> TPTTFVHLFEWNWQDVAQECEQYLGPKGYAAVQVSPPNEHITGSQWWTRYQPVSYELQSRGGNRAQFIDMVNRCSAAGVDIYVDTLINHMAAGSGTGTAGNSFGNKSFPIYSPQDFHESCTINNSDYGNDRYRVQNCELVGLADLDT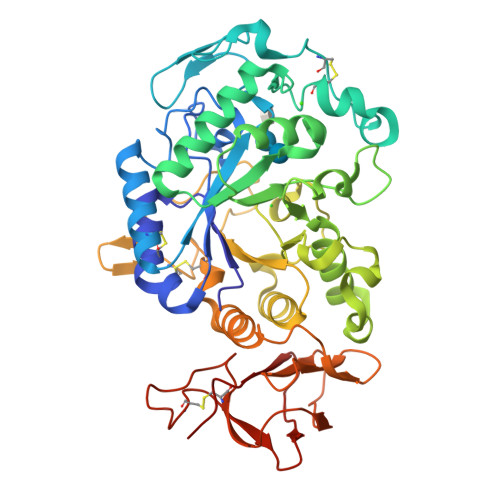ASNYVQNTIAAYINDLQAIGVKGFRFNASKHVAASDIQSLMAKVNGSPVVFQEVIDQGGEAVGASEYLSTGLVTEFKYSTELGNTFRNGSLAWLSNFGEGWGFMPSSSAVVFVDNHDNQRGHGGAGNVITFEDGRLYDLANVFMLAYPYGYPKVMSSYDFHGDTDAGGPNVPVHNNGNLECFASNWKCEHRWSYIAGGVDFRNNTADNWAVTNWWDNTNNQISFGRGSSGHMAINKEDSTLTATVQTDMASGQYCNVLKGELSADAKSCSGEVITVNSDGTINLNIGAWDAMAIHKNAKLN N-[(2S)-1-hydroxypropan-2-yl]butanamide | C7 H15 N O2 | 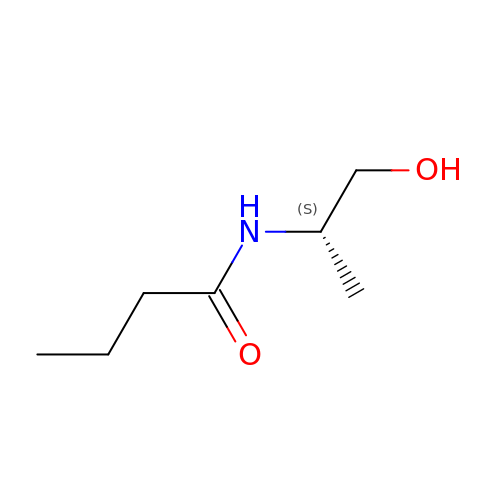LQLCVBWKNBEZHW-LURJTMIESA-N>[2x]AGHSTQTAEDKEEPLHSIISSTESVQGSTSKHEFQAETKKLLDIVARSLYSEKEVFIRELISNASDALEKLRHKLVSDGQALPEM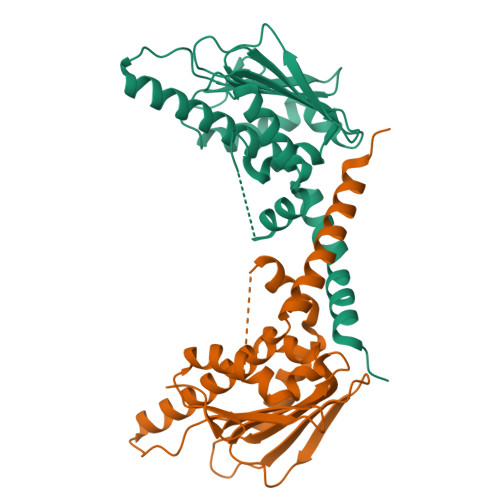EIHLQTNAEKGTITIQDTGIGMTQEELVSNLGTIARSGSKAFLDALQNQAEASSKIIGQFGVGFYSAFMVADRVEVYSRSAAPGSLGYQWLSDGSGVFEIAEASGVRTGTKIIIHLKSDCKEFSSEARVRDVVTKYSNFVSFPLYLNGRRMNT>MKKEKNCLRIYWGIYQHLQGNDLLEDSPYEPVNSRLSDIFRLAPIYSGEPALAKENNCLNAAKACNLNDTCKKYRSAYISPCTSRVSTAEVCNKRKCHKALRQFFDKVPPKHSYGMLYCSCPLGDQSACSERRRQTIVPACSYEDKERPNCLTLQVSCKTNYICRSRLADFFTNCQPEPLSLSGCLKENYADCLLSYSGLIGTVMTPNYLRSPKISVSPFCDCSSSGNSKEECDRFTEFFTDNACLRNAIQAFGNGTGSE[10x];>GQGRGCLLKEIHLNVTDLDLGYRTKEELIFRYCSGPCHDAETNYDKILNNLTHNKKLDKDTPSRTCCRPIAFDDDISFLDDSLEYHTLKKHSAKKCACV[10x]

Glial-cell line derived neurotrophic factor (GDNF) bound to its co-receptor GFRα1 stimulates the RET receptor tyrosine kinase, promoting neuronal survival and neuroprotection. The GDNF-GFRα1 complex also supports synaptic cell adhesion independently of RET. GFRα family members consist of either two or three extracellular cysteine-rich helical domains (D1-3) followed by a flexible C-tail (CT) and either a glycophosphatidylinositol (GPI)-anchor or a transmembrane domain (GFRAL). Each GFL-GFRα complex has a 2:2 stoichiometry (GFL2-GFRα2) that adopts a U-shaped structure with variable hinge angles.

Here, we describe the structure of a decameric GDNF-GFRα1 assembly determined by crystallography and electron microscopy, revealing two GFRα1 pentamers bridged by five GDNF dimers. The monoclinic crystals were grown using recombinant zGFRα1 residues 20-353, (defined as zGFRα1D1-D3, lacking the GPI-anchor) in complex with zGDNF residues 134–235 (mature form of GDNF, defined hereafter as zGDNFmat). Missing from the structure is the zGFRα1 D1 domain, which we found to be removed by time-dependent proteolytic clipping during crystallisation. Within the decameric assembly, the five ‘U’-shaped GDNF2-GFRα12 sub-complexes associate with one another about the five-fold axis through GFRα1:GFRα1 interactions from the tips of the ‘U’. This arrangement generates two GFRα1 pentamer rings (green in Fig. 1b) that form the base and lid of the barrel, connected by five covalent GDNF dimer ‘staves’ (yellow/orange in Fig. 1b). The barrel molecular dimensions are 138 Å in length with a diameter of 118 Å. Unique to the barrel however, is a homophilic GFRα1:GFRα1 interface generated by the non-crystallographic five-fold rotational symmetry. To form this interface, helices α12 and α15 from the D3 domain of one GFRα1 molecule (grey in Fig. 1d) dock into a groove formed by helix α9, helix α14 and helix α16 in the adjacent GFRα1 protomer (green in Fig. 1d). The interface includes L247/V251 from helix α12, L289/L290 from helix α14 and F348 from helix α16, together with several hydrogen bonds and charge interactions at the interface periphery. Electron density can be seen extending from the specific N-glycosylation site of all zGDNF protomers and a total of 8 N-linked glycans for the 10 zGFRα1 protomers are well resolved within the barrel structure.>[2x]GMAADILVVDDEVDIRDLVAGILSDEGHETRTAFDADSALAAINDRAPRLVFLDIWLQGSRLDGLALLDEIKKQHPELPVVMISGHGNIETAVSAIRRGAYDFIEKPFKADRLILVAERALETSKLKREVSDLRKRTGDQLELVGTSLAMNQLRQTIERVAPTNSR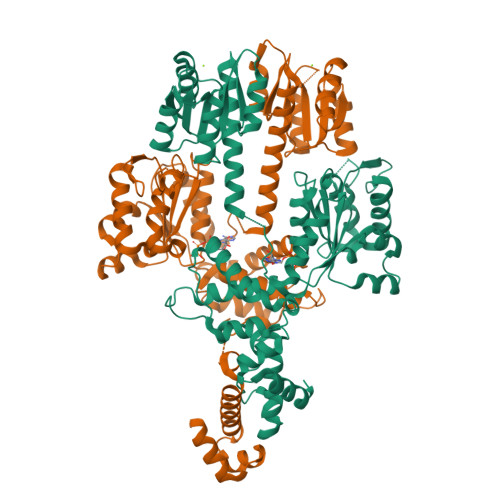IMITGPSGAGKELVARAIHAQSSRANGPFVTVNAATITPERMEIELFGTEMDGGERKVGALEEAHGGILYLDEVADMPRETQNKILRVLVDQQFERVGGTKRVKVDVRIISSTAQNLEGMIAEGTFREDLFHRLSVVPVQVPALAARREDIPSLVEFFMKQIAEQAGIKPRKIGPDAMAVLQAHSWPGNLRQLRNNVERLMILTRGDDPDELVTADLLPAEIGDTLPRAPTESDQHIMALPLREARERFEKEYLIAQINRFGGNISRTAEFVGMERSALHRKLKSLGV3-methyl-N-[(1R)-1-(1H-1,2,4-triazol-3-yl)ethyl]-4-{1-[6-(trifluoromethyl)pyridin-3-yl]cyclopropyl}-1H-pyrrole-2-carboxamide | C19 H19 F3 N6 O | 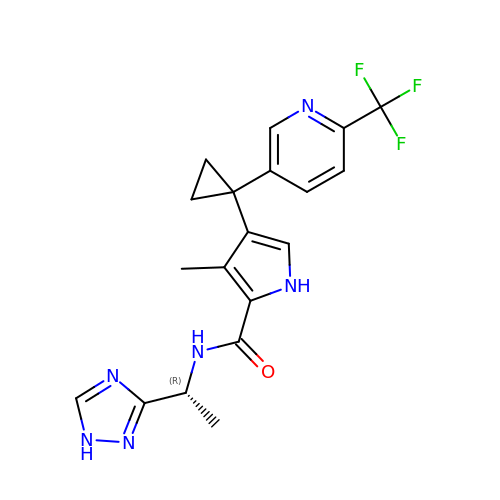JUBPRXDFKLPILK-LLVKDONJSA-N>[3x]IGATEQSYVASAVTPLRLNSSTKVLDMLIDSSTLEINSSGQLTVRSTSPNLRYPIADVSGGIGMSPNYRFRQSMWIGIVSYSGSGLNWRVQ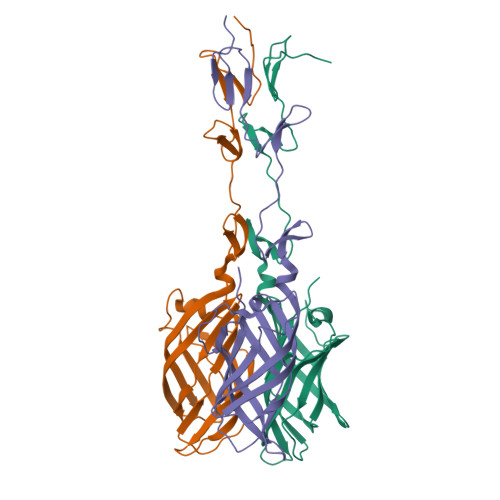VNSDIFIVDDYIHICLPAFDGFSIADGGDLSLNFVTGLLPPLLTGDTEPAFHNDVVTYGAQTVAIGLSSGGAPQYMSKNLWVEQWQDGVLRLRVEGGGSITHSNSKWPAMTVSYPRSFT hMcl-1 is often overexpressed in cancer, where it confers resistance to chemotherapy or radiation. In the current work, we created novel stapled peptides that are intended to target hMcl-1 His 252 covalently. However, two His residues, namely, His 252 and His 224, are present in the BH3 binding pocket of Mcl-1 and could be therefore targeted perhaps more efficiently with covalent agents compared to Lys 234. His residues are particularly attractive yet underexplored for covalent drug design given that they, unlike Lys, are usually unprotonated at physiological pH, which should facilitate a nucleophilic addition at the imidazole ring.

Based on previous experience with hMcl-1(172–323) and with an artificial model system, we used to assess covalent His targeting, we introduced a 2-methoxy 5-sulfonyl fluoride on the side chain of a 3 amino propionic acid to introduce the possible electrophile for His/Lys covalent adduct formation, in addition to constraining the alpha-helix with chemical staples at various positions. To further elucidate the binding conformation of the covalent agent to hMcl-1(172–323) and to more unambiguously identify the covalently targeted residue, we determined the X-ray structure of compound 155H1 in complex with hMcl-1(172–323). As anticipated by previous characterizations, we found that the N-terminal residue formed a covalent bond with the side chain of His 252, as observed by a contiguous electron density between the aryl-sulfonyl group and the imidazole ring of His 252 with whom the group formed a stable sulfonamide. In the final refined model, the density and placement of covalently bound 155H1 in the hMcl-1(172–323) structure were well resolved in its entirety. The general peptide-hMcl-1(172–323) interactions appeared well maintained in the crystal structure, in which the amphipathic helical peptide was inserted into the peptide-binding pocket with its hydrophobic side chains buried in the pocket, while the peptide’s only Asp residue was involved in a salt bridge with hMcl-1(172–323) residue Arg 263. These interactions are typically well conserved between BH3 peptides and hMcl-1(172–323)12 as well as in other BH3/Bcl-2 protein complexes. The data, however, suggest that His 252 is the likely target for our agents, given that the covalent adduct formation was detected with both wt and the Lys234Ala hMcl-1(172–323) mutant. However, as anticipated earlier, the agents can also interact covalently with Lys 234 when His 252 was mutated to Ala. However, when the protein was exposed to stapled covalent agent 155H1, resonances of the binding site His 224 further broadened beyond detection, while the cross-peaks for the imidazole resonances of His 252 were dramatically shifted for all 3 observed resonances, presumably due to the formation of the covalent adduct with His 252. Likewise, a shift in the band was also appreciable when intact A549 cells were exposed to 155H1.

> GSHMDELYRQSLEIISRYLREQATGAKDTKPMGRSGATSRKALETLRRVGDGVQRNHETAFQGMLRKLDIKNEDDVKSLSRVMIHVFSDGVTNWGRIVTLISFGAFVAKHLKTINQESCIEPLAESITDVLVRTKRDWLVKQRGWDGFVEFFHVED;> XAIAEQLRAIGDAFX> NLYQFKNMIQCTVPSRSWAD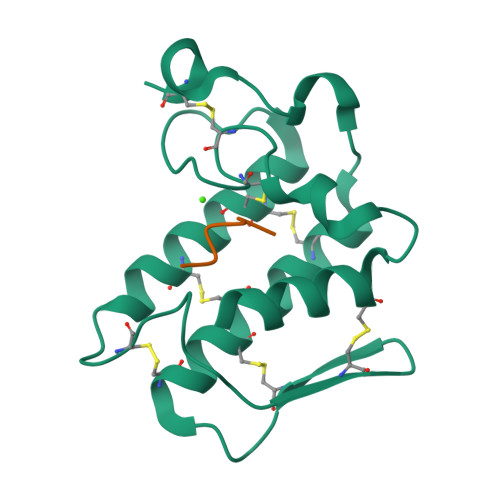FADYGCYCGKGGSGTPVDDLDRCCQTHDNCYNEAENISGCRPYFKTYSYECTQGTLTCKGDNNACAASVCDCDRLAAICFAGAPYNDANYNIDLKARCN;> KLVFFA>[2x]NSDSECPLSHDGYCL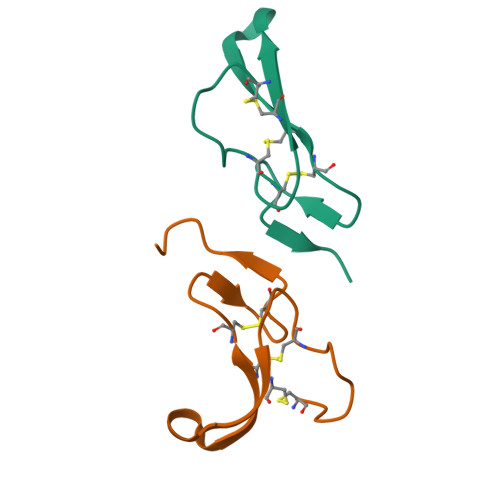HDGVCMYIEALDKYACNCVVGYIGERCQYRDLKWWE>[12x]MHHHHHHGGGGGMPTSPSKKLVVLDRDGVINVDSDAFVKSPDEWVALPGSLEAIARLNHAGYRVVVATNQSGIGRGLFDMATLNAM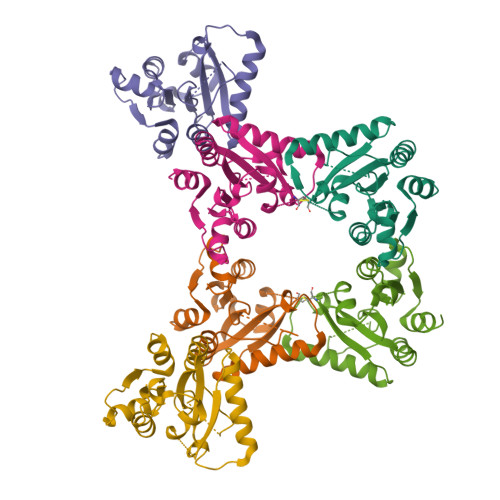HLKMHRAAAAVGGRIDAVFFCPHTADDHCDCRKPMPGMMKLIAERFEIDPADTPVVGDSLRDLQAGAALGFRPHLVLTGKGKKTLAAGGLPEGTRVHDDLRAFALDFLSKEHE> MERPESELIRQSWRVVSRSPLEHGT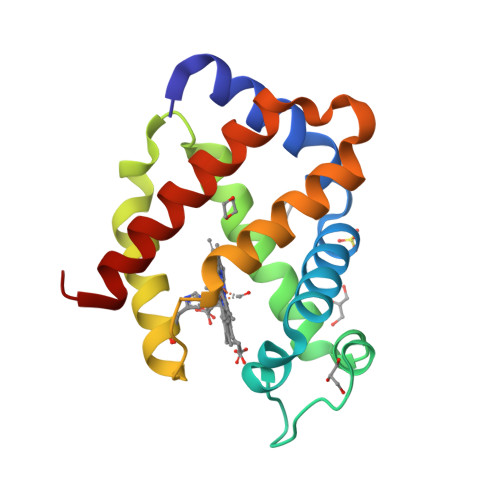VLFARLFALEPSLLPLFQYNGRQFSSPEDSLSSPEFLDHIRKVMLVIDAAVTNVEDLSSLEEYLTSLGRKHRAVGVRLSSASTVGESLLYMLEKSLGPDFTPATRTAWSRLYGAVVQAMSRGWDGE> MAMPDVQYPINTYGWLKKAVALWADRDDDEFVNQIPNFINFAEKEIYRNLRIPPLEKEVYLDIKDGVAYIPPDYLEAQWMMRAKDGTIFQVTSPEEISYRRQHGTINPSHWNNQPVNFARFGSRFIFYPSIEADTPYYPDDGSPLIPAENSVILSYYADPPEFHEDTDTSTILTIAPELLLYFTLRHACLFVQDDNGVQK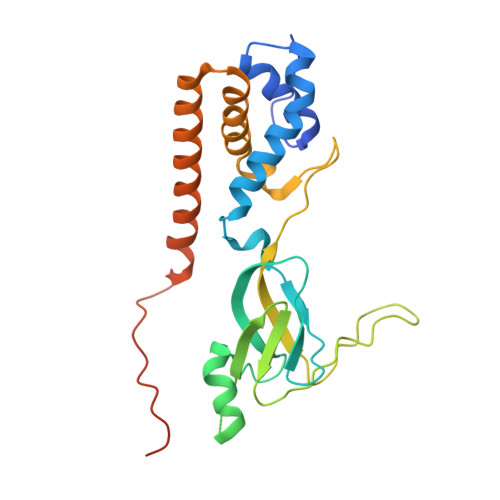WSALGKAILDEMVEQNKKQEYSGSPIAIPNNMTRLQSSLPDIYGIRTSRV> MFRISLICFPKAGCEEITRQGRRVVLKPQEYFAQHRMQVWQMRFKEMGPPFSRVWVALGGKMRRRRIGRQIDVKDMRYYWRPIEPQYQRLYMSRLRIKDHSNKRVQPMRLRATNNDIGQASSLKEWERSSDRKYGAALAPP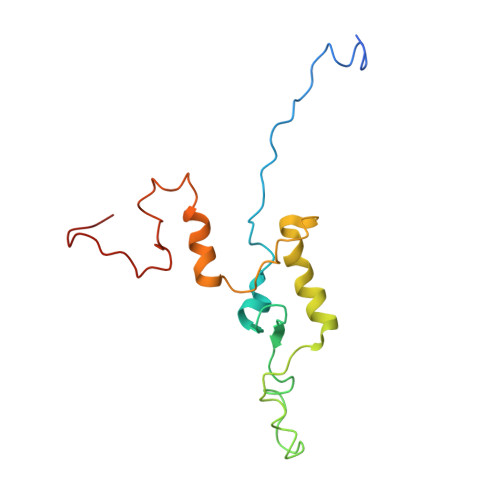KKRDFEFRVF>[4x]MDHHHHHHLPNITILATGGTIAGGGDSATKSNYTVGKVGVENLVNAVPQLKDIANVKGEQVVNIGSQDMNDNVWLTLAKKINTDCDKTDGFVITHGTDTMEETAYFLDLTVKCDKPVVMVGAMRPSTSMSADGPFNLYNAVVTAADKASANRGVLVVMNDTVLDGRDVTMTNTTDVATFKSVNYGPLGYIHNG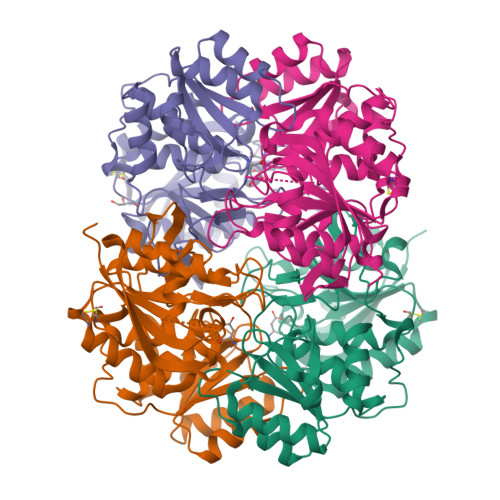KIDYQRTPARKHTSDTPFDVSKLNELPKVGIVYNYANASDLPAKALVDAGYDGIVSAGVGNGNLYKSVFDTLATAAKTGTAVVRSSRVPTGATTQDAEVDDAKYGFVASGTLNPQKARVLLQLALTQTKDPQQIQQIFNQY5-[[(2R)-7-fluoranyl-2-phenyl-2,3-dihydrothieno[3,2-b]indol-4-yl]methyl]-N-oxidanyl-thiophene-2-carboxamide | C22 H17 F N2 O2 S2 | 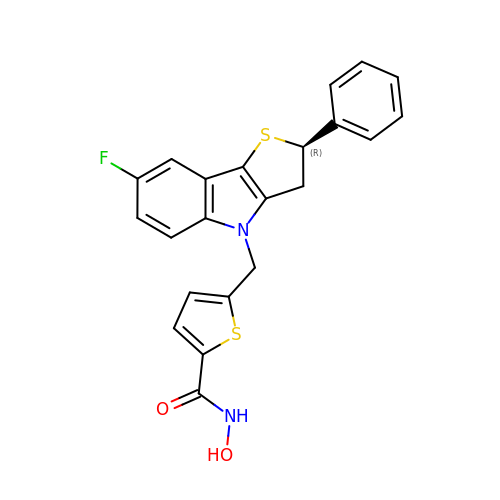IGIBSWIQIIJZKL-HXUWFJFHSA-N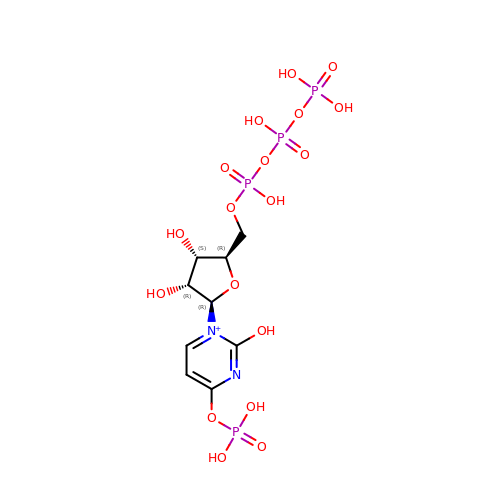[[(2~{R},3~{S},4~{R},5~{R})-3,4-bis(oxidanyl)-5-(2-oxidanyl-4-phosphonooxy-pyrimidin-1-yl)oxolan-2-yl]methoxy-oxidanyl-phosphoryl] phosphono hydrogen phosphate | C9 H17 N2 O18 P4 | RYGLMDXZXSWNKW-XVFCMESISA-O> MADYKDDDDKSGPDEVDASGRMAGMALARAWKQMSW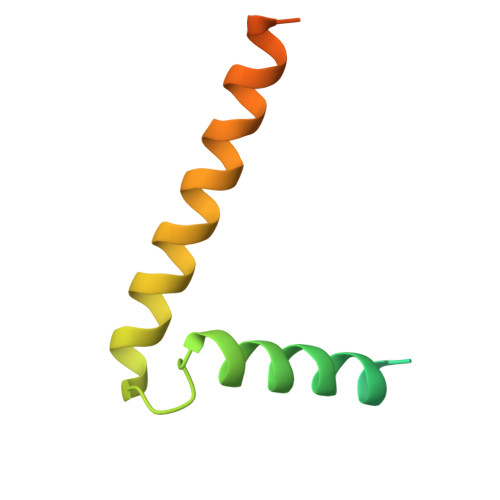FYYQYLLVTALYMLEPWERTVFNSMLVSIVGMALYTGYVFMPQHIMAILHYFEIVQ> CGYIPTSKIANNIFDEKVYVNVELSQQDPKNSIYVADTLKEMVISKLGRKLALKHEADDVINVKMNNLEFIPLAYDKNGYVISYKAKLNLDFNVVFKDGSSQAFSTSGSYNFE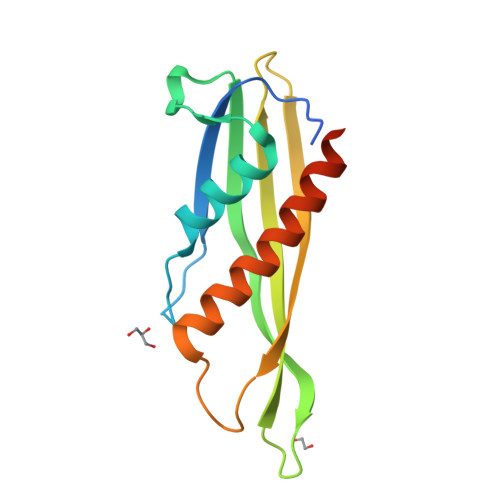ISPNSIISDSARYEAIRAASSEAFDEFISVIAIKGQKRDSKY>[2x]TTEKRNRNLLYEYAREGYSALPQLDIERFCACPEEAAHALELRKGELRSADLPAIISTWQELRQLQEQIRSLEEEKAAVTEAVRALLANQDSGEVQQDPKYQGLRARGREIRKELVHLYPREAQLEEQFYLQALKLPN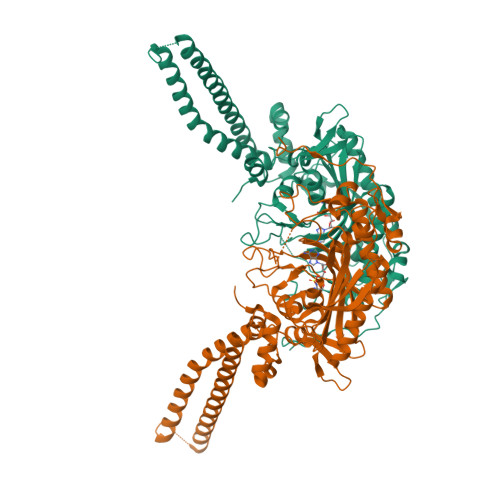QTHPDVPVGDESQARVLHMVGDKPVFSFQPRGHLEIGEKLDIIRQKRLSHVSGHRSYYLRGAGALLQHGLVNFTFNKLLRRGFTPMTVPDLLRGAVFEGCGMTPNANPSQIYNIDPARFKDLNLAGTAEVGLAGYFMDHTVAFRDLPVRMVCSSTCYRAETNTGQEPRGLYRVHHFTKVEMFGVTGPGLEQSSQLLEEFLSLQMEILTELGLHFRVLDMPTQELGLPAYRKFDIEAWMPGRGRFGEVTSASNCTDFQSRRLHIMFQTEAGELQFAHTVNATACAVPRLLIALLESNQQKDGSVLVPPALQSYLGTDRITAPTHVPLQYIGPNQPRKPGLPGQPAVS> MGSSHHHHHHSS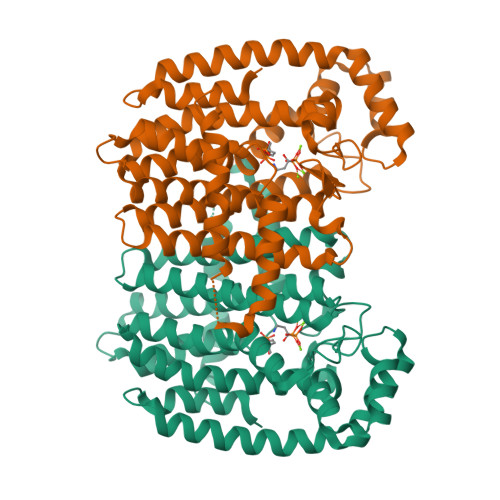GRENLYFQGHMNGDQNSDVYAQEKQDFVQHFSQIVRVLTEDEMGHPEIGDAIARLKEVLEYNTIGGKYNRGLTVVVAFRELVEPRKQDADSLQRAWTVGWCVELLQAFFLVADDIMDSSLTRRGQICWYQKPGVGLDAINDANLLEACIYRLLKLYCREQPYYLNLIELFLQSSYQTEIGQTLDLLTAPQGNVDLVRFTEKRYKSIVKYKTAFYSFYLPIAAAMYMAGIDGEKEHANAKKILLEMGEFAQIQDDYLDLFGDPSVTGKIGTDIQDNKCSWLVVQCLQRATPEQYQILKENYGQKEAEKVARVKALYEELDLPAVFLQYEEDSYSHIMALIEQYAAPLPPAVFLGLARKIYKRRK> MGSSHHHHHHSQDPMEIDELTALGGLLHDIGKPVQRAGLYSGDHSTQGARFLRDLAENTGRAEYELLSLFSEFHHKGHMKNDELMIRRIKELSPERFGLTMEDVLNALWIVYEADNLASGEREEGQPQASRPLYSVFNPGKAYPWAELDFEKELPVPGDVFSIRSQDYRELVKRLWEELSKAKLRSDRLLPVLEKYLTFVSSVTSEGNIISLYDHMRMTSAIALAMLRAGCTAEDVRSGRCRKEKRFLLIEGDFSGIQDFIYRVSGKGTLKYLRARSAYLELIGWDVVLEILSRLGLTRANVVFNAGGHFMIIAQNTPDAVKELEEIRAKAVEWLYREFESDLYLAIEWEPVSGREFGREGGKNLFAEARKRLKHKLTVRKLKRFGEIKGLFEHGHTERLAECPVCGRELPEGKLEPSASDPETKVCPTCNRLVSLGGNLPKLLGFGRTAKNDAGVLVEGPFSGFVPYLQGGRPVGEQILVKNTLNPGEIPESAQFVPYFVADYFKKDPKGGVATFEELSMASTGTRRLGVMKGDVDRLGEFFSSMDSPSKLATASRFMDYFFKGYIGAIIEGKFGYIIGDVPSLRDWPEEPDIVVVYAGGDAFFIVGAWDQIFELAFRVRRAFNAYTGGKLTLSVGLGYFDERTPIYRMADVVSERLDTAKDEGRNRVFVVGRSRPLDGKHKLSYEWNHYEELWRTYAPRIYAGNGRLKGKLESKKGLLWKLLEIRELYVRDPNDVRWAYLTAYLLGRHGLSDLFPELVGIDT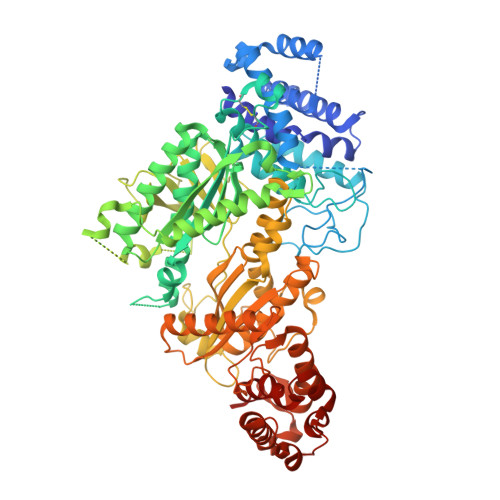KAVERKEPQPVYWVDGVLKIVLMAVRR>GSMPLLLDDGDPKAQTGFDLSTATTLFWRPVPVHVKQQDREDVLEELTFRILTGVAKQNHNLRILRIHISSDSDLFFLHTLEVSEEDFQSLKNDEGILVDF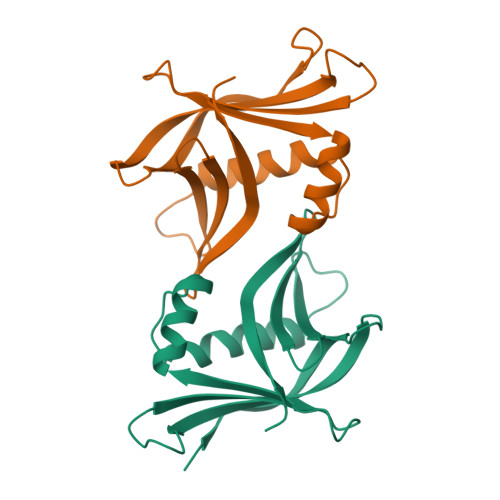ASFPGKIISLLEKCILAQPGDSPRFQAVLTIRGGESVFKIVEINDFKQLPHITLAFRPGN[2x]> MDLIGRGGAPSASALGTDALVLLCGPEAQAGISTCSAAAESAASPQSSCSWVGTAQHSSATRAEAAGPSAPCGPAPLLRNLRTPSQSGRLSGAPPTWISAAAASLGNSPRFAASARCSTADVDVSRSGLEDASALGDCVDRWSTPAATVSGIALLHQYHNHHHNHHHIGHSSSSCGSVASSTSSVPGSAAGSPFPPRPSLPSSATNSSRFLMQSQSQQLRSVSFTAATAAPKAAAKGASAKAGSSSSSGAAAPSPAAAALRTPEWARVPGHLHELQDLYRKRQKRMAALRHGAQVELEAREAVAWKTGGRGRAVAAAAKAALDALPLPPPEDGGKAELAAALAADTTFAAAHEALTGLLRRGVVLDAAEHLAPLLRKAGDAGQLASALGVA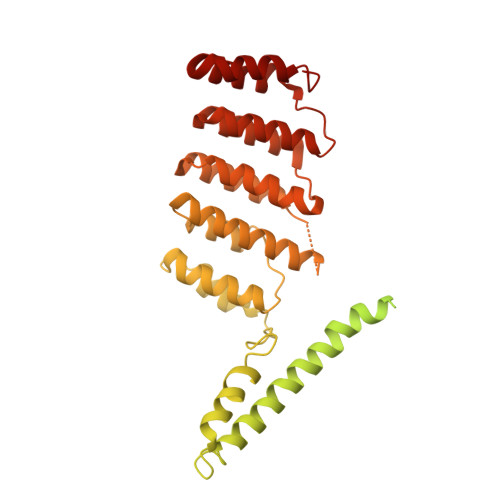AANHLSQAARQLGAHSPRHGPLHAVLVQECRRLKAAAPLVTLWESLHEHGLAPEAADAAAAVRAAVELGDGGAAVRLLMLACMYGEAPLAGAAEAGAVLQLLQQGNPDQAAQLRELLPKLGLRGA>GMVEQRNRGRPAVPDAVVRESIVGAAQRLLSSGGAAAMTMEGVASEAGIAKKTL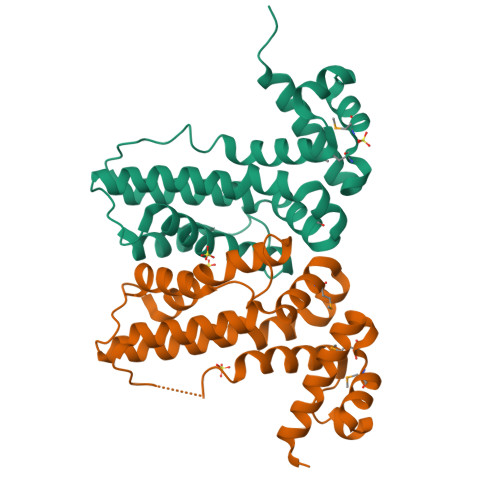YRFASGRADLIGLLVESWIAPIFPGFEADPQDAAAALERIVYDIAQAVLSREAVSLFRMLASDADLRNRFLPAYNANGIERSRRELARWLDQQASAGRLPLPIPAERVADLLLSAVIAEPLRQITLGLREPLPAWDIAPRVADAVRLIAPGRER[2x]> MGHHHHHHHHHHSSGHIEGRHMFSKNAVKLHATPPSVAAPPTGAPEVAAERLEPRVEEKDGYWILKEQFRKGINPQEKVKIEKEPMKLFMENGIEELAKIPIEEIDQSKLTKDDIDVRLKWLGLFHRRKNQYGRFMMRLKLPNGVTTSAQTRYLASVIRKYGKEGCADITTRQNWQIRGVVLPDVPEILKGLAEVGLTSLQSGEDNVRNPVGNPLAGIDPEEIVDTRPYTNLLSQFITGNSRGNPAVSNLPRKWNPCVVGSHDLYEHPHINDLAYMPATKDGRFGFNLLVGGFFSAKRCDEAIPLDAWVPADDVVPVCRAILEAFRDLGFRGNRQKCRMMWLIDELGVEGFRAEVEKRMPQQQLERASPEDLVQKQWERRDYLGVHP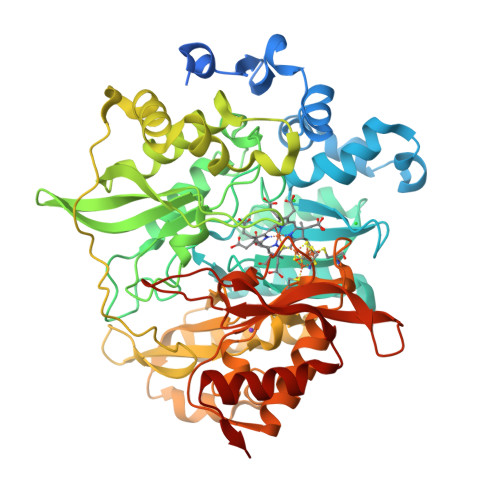QKQEGYSFIGLHIPVGRVQADDMDELARLADEYGSGEIRLTVEQNIIIPNIETSKIEALLKEPVLSTFSPDPPILMKGLVACTGNQFCGQAIIETKARSLKITEEVQRQVSLTKPVRMHWTGCPNTCAQVQVADIGFMGCLTRDKNGKTVEGADVFLGGRIGSDSHLGEVYKKAVPCDDLVPLVVDLLVNNFGAVPR> MSHPIQFVNANNSDKSHQLGGQYSIPQDLRENLQKEAARIGENEKDVLQEKMETRTVQNREDSYHKRRFDMKFEPDSDTQTVTSSENTQDAVVPRKRKSRWDVKGYEPPDESSTAVKENSDSALVNVEGIHDLMFFKPSDHKYFADVISKKPIDELNKDEKKERTLSMLLLKIKNGNTASRRTSMRILTDKAVTFGPEMIFNRLLPILLDRSLEDQERHLMIKTIDRVLYQLGDLTKPYVHKILVVAAPLLIDEDPMVRSTGQEIITNLSTVAGLKTILTVMRPDIENEDEYVRNVTSRAAAVVAKALGVNQLLPFINAACHSRKSWKARHTGIKIVQQIGILLGIGVLNHLTGLMSCIKDCLMDDHVPVRIVTAHTLSTLAENSYPYGIEVFNVVLEPLWKGIRSHRGKVLSSFLKAVGSMIPLMDPEYAGYYTTEAMRIIRREFDSPDDEMKKTILLVLQKCSAVESITPKFLREEIAPEFFQKFWVRRVALDRPLNKVVTYTTVTLAKKLGCSYTIDKLLTPLRDEAEPFRTMAVHAVTRTVNLLGTADLDERLETRLIDALLIAFQEQTNSDSIIFKGFGAVTVSLDIRMKPFLAPIVSTILNHLKHKTPLVRQHAADLCAILIPVIKNCHEFEMLNKLNIILYESLGEVYPEVLGSIINAMYCITSVMDLDKLQPPINQILPTLTPILRNKHRKVEVNTIKFVGLIGKLAPTYAPPKEWMRICFELLELLKSTNKEIRRSANATFGFIAEAIGPHDVLVALLNNLKVQERQLRVCTAVAIGIVAKVCGPYNVLPVIMNEYTTPETNVQNGVLKAMSFMFEYIGNMSKDYIYFITPLLEDALTDRDLVHRQTASNVITHLALNCSGTGHEDAFIHLMNLLIPNIFETSPHAIMRILEGLEALSQALGPGLFMNYIWAGLFHPAKNVRKAFWRVYNNMYVMYQDAMVPFYPVTPDNNEEYIEELDLVL;> MWGGGKMAVVSLSPHTAKMRKLFGQASTTMAYDGLKREAERRTRSDHNITMVAKDDELYLYHLTLKKQTNFVHSCIGHFVDLEAGSKREQSQLCVATETHLELYDTADGELKLIAKFQNLFATITSMKSLDLPHSGSRAKASNWPTFLALTSDSGNLSIVQIIMHAGALRLKTLVNQPLTRTTLRRVSPISYMEIDPNGRCIILSSVEQNKLCFLVDYAQKLRISSPLEIIRPHMVTLDMAVVDVNFNNPCFVTLEIDNAATQLSVHLIFYVLELGLNHIVKKADYLVNPSANFVLSLPDLSRYNITTSLSDNNYDADYDTLFNPFVVIGFENHILVKDMNGFFSLKVEIPKRSITNSRHKNVTIISGIVQKLKNDFFVLLQSNHGDLFKLTVSPDTNDRNRPLVQLSYFDTIQNSHQLHIFKNGYLFALSEMNNNFLFQFEKLGVEKNDFSNVLTSKDPNKSLVFEPSIKLQNLSILSQQLNLNPSIKSQIVSDSPLSIATKHFTNNKIITLTNAVNYSNLISTSLPPNATKLWLIPDPATTGDNNTLLFITFPKKTMILQIDNESMEELTPDEATRSAFKLSQDTTIHTCLMGSHSIIQVCTAELRHIVPTGKSRYSNKLTWVPPAGIRIVCATSSKTQLIISLSNYELVYFKIDVSSDSLIELTTHPELDTMPSKVAIVQDTQHADLLAIADNEGMIKIMSLKDQKEDFLTVISLQLVSEKISDMIMVRDSSIGQLNLHVGLENGVYMKFHIGDVDGSFTDIKRRFLGLKPVSLSYLREISVSLNNEEEEEEEEDDDDEKEEEEINSSGAKWMSCVVCHSSSTWVSYTWKNVWTIRQLKDQNMLSCSKFVNADVAINGVCSISSSGRLNIGRVSNFPTLDNWFHVHESSVNKQENGGGDESNEEEEDEMEEEMEMLQISTFRPRTILSFPNNPKSILFIDNHSGKKQCRISLQIDGECLKFGSSDHLYKILDDIDCVSAAIIDFTRQADHLIICAGDKRLLTYKILVNKDKLSFDIELLHQTEIISPIHAMLKFKNFLLTAMGSTIVLYGLGKKQLLRRSVTQTPVSITKIVSMHQWNYERLAVGDIHESVTLFIWDPAGNVFIPYVDDSVKRHVTVLKFLDEATVIGADRYGNAWTLRSPPECEKIMSNHDPSELSNGAIKYPLDVITLQQKLPNTYDCKFKFQLLNHFFVNDIITDFHILDSLSNSDRPGCIYMGLQGTVGCFIPLLSKGNVFMMGNIENIMAEADDTFYLDYESRKKNNNMRKEDDEEESGSVVLQGRHGIEDEIICEGSCSILGRDHQEYRSYYAPVRKVIDGDLCENFLRLSLNEQEFLAKNLKSVQVEDIIQTINEVRTNYM;> MARTKSRKRSGNNQNKNASVVNNKAEIAAMIDARRLEQKKKGGVTNSKGKTNKVVDAKLEKEFKDVLQRFQVQENDTPKEITKDEKNNHVVIVEKNPVMNRKHTAEDELEDTPSDGIEEHLSARKRRKTEKPSLSQLKSQVPYPQIIEWYDCDARYPGLLASIKCTKNVIPVPSHWQSKKEYLSGRSLLGKRPFELPDIIKKTNIEQMRSTLPQSGLDGQDEKSLKEASRARVQPKMGALDLDYKKLHDVFFKIGANWKPDHLLCFGDVYYENRNLFEETNWKRMVDHKRPGRISQELRAIMNLPEGQLPPWCMKMKDIGLPTGYPDLKIAGLNWDITNLKGDVYGKIIPNHHSRSKKQGRNYFGALISFETPEFENSKEDTQANAENGRQDDKIDDEVEHKLDHFQEDISEVTSAEEKLERNEEESEKQLYTVLK;> MNYSADSGNTVYVGNIDPRITKEQLYELFIQINPVLRIKYPKDKVLQAYQGYAFIEFYNQGDAQYAIKIMNNTVRLYDRLIKVRQVTNSTGTTNLPSNISKDMILPIAKLFIKNLADSIDSDQLVKIFNKFGKLIREPEIFYLSNGKLKCAYVYFEDFEKADLAIKSLNNQLVANNRITVDYAFKENGKGNAKYGDDVDRLLNKEALKHNMLK;> MSRHQFDLIMCLKQPGVQTGLLCEKCDGKCPICDSYVRPKRKVRVCENCSFGKQAKNCIICNLNVGVNDAFYCWECCRLGKDKDGCPRILNLGSNRLDRHFEKKKKV;> MNLLETRRSLLEEMEIIENAIAERIQRNPELYYHYIQESSKVFPDTKLPRSSLIAENKIYKFKKVKRKRKQIILQQHEINIFLRDYQEKQQTFNKINRPEETQEDDKDLPNFERKLQQLEKELKNEDENFELDINSKKDKYALFSSSSDPSRRTNILSDRARDLDLNEIFTRDEQYGEYMELEQFHSLWLNVIKRGDCSLLQFLDILELFLDDEKYLLTPPMDRKNDRYMAFLLKLSKYVETFFFKSYALLDAAAVENLIKSDFEHSYCRGSLRSEAKGIYCPFCSRWFKTSSVFESHLVGKIHKKNESKRRNFVYSEYKLHRYLKYLNDEFSRTRSFVERKLAFTANERMAEMDILTQKYEAPAYDSTEKEGAEQVDGEQRDGQLQEEHLSGKSFDMPLGPDGLPMPYWLYKLHGLDREYRCEICSNKVYNGRRTFERHFNEERHIYHLRCLGIEPSSVFKGITKIKEAQELWKNMQGQSQLTSIAAVPPKPNPSQLKVPTELELEEEDEEGNVMSKKVYDELKKQGLV;> MNYLEGVGSKKGGGGIASESQFNLQRRKEVESLLSKGENVPYTFQDEKDDQVRSNPYIYKNHSGKLVCKLCNTMHMSWSSVERHLGGKKHGLNVLRRGISIEKSSLGREGQTTHDFRQQQKXXXXXXXXXXXXXXXXIIEAKQSLKNNGTIPVCKIATVKNPKNGSVGLAIQVNYSSEVKENSVDSDDKAKVPPLIRIVSGLELSDTKQKGKKFLVIAYEPFENIAIELPPNEILFSENNDMDNNNDGVDELNKKCTFWDAISKLYYVQFFFKQAEQEQADV;> MEPEDTQLKEDIKTTVNYIKQHGVEFENKLLEDERFSFIKKDDPLHEYYTKLMNEPTDTVSGEDNDRKSEREIARPPDFLFSQYDTGISRRDMEVIKLTARYYAKDKSIVEQMISKDGEARLNFMNSSHPLHKTFTDFVAQYKRVYSFTGQEIKKSKRTILDNCFERTQYWEFEKDKDREHDKLVELCKIQFAAIPWDKFTQVAKFSIPEDTEIFEGSLDLEQMRLRRVQTGIKLFDSIKPTNEEEKIVSDQGKQKGGDSKGKKRKIRAVGETRLKKSKK;> MKFTPSIVIDAPQYYVDHFNGKYNVDKCVILRDLQLETDSESMPSSLKHLTKPTHILDLTNNDLIMIPDLSRRDDIHTLLLGRNNIVEVDGRLLPMNVQNLTLSNNSIRRFEDLQRLRRAPRTLKNLTLIGNQVCHLANYREHVLRLVPHLETLDFQNVTAEERKSAMSFPRQADGDTLGPVNTAIRDNGSRDKTMEIMNLVVSKMTVERRNELKKQLAEATSLEEIARLEKLLSGGV;> MVEPARKKQRIDRDTHHTVAEPVTEAKNTLYVSQLNEKINMQRLRVNLFLLFATFGEVLKVSMNFKKQRGQAFITMRTIDQASLAQISLNGERFFGKPLKVEFSKSETKTL;> MAEKQRQLKLQKIYKQKYIGLGDESTTREQWQRNVRNDTLNTLQGHSASLEYVSLSRGDLSIRDTRIHLLKSMSPGYKAYLREE;> METIDSKQNINRESLLEERRKKLAKWKQKKAQFDAQKEHQTSRNDIVTNSLEGKQTTEKFTERQERVKEELRKRKNEFRKSDEPVSVKPSKKKSKRSKVKKKISFDFSDDDDSEIGVSFRSKEHIQKAPEHDNEKDPLDEFMTSLKEEKMSNSKGMYDRGDILDVEDQLFELGGTDDEDVEDNTDNSNIAKIAKLKAKKRVKQIYYSPEELEPFQKNFYIESETVSSMSEMEVEELRLSLDNIKIKGTGCPKPVTKWSQLGLSTDTMVLITEKLHFGSLTPIQSQALPAIMSGRDVIGISKTGSGKTISYLLPLLRQVKAQRPLSKHETGPMGLILAPTRELALQIHEEVTKFTEADTSIRSVCCTGGSEMKKQITDLKRGTEIVVATPGRFIDILTLNDGKLLSTKRITFVVMDEADRLFDLGFEPQITQIMKTVRPDKQCVLFSATFPNKLRSFAVRVLHSPISITINSKGMVNENVKQKFRICHSEDEKFDNLVQLIHERSEFFDEVQSENDGQSSDVEEVDAKAIIFVSSQNICDFISKKLLNAGIVTCAIHAGKPYQERLMNLEKFKREKNSILLCTEVLSRGLNVPEVSLVIIYNAVKTFAQYVHTTGRTARGSRSGTAITLLLHDELSGAYILSKAMRDEEIKALDPLQAKELQEMSAKFESGMKKGKFRLSKGFGGKGLENIKSKREEAQNKDLELKKNDKRSDDLEKKISNPREGHDSVSESSALIPRLNYELFKESTDGSIIFYAKVYINDLPQIVRWEATKNTTLLFIKHETGCSITNKGKFYPEGKEPKNENDEPKLYLLIEGQDEKDIQLSIELLEQKVKEGVVKAASLSLKSTKY;> MSKIQVAHSSRLANLIDYKLRVLTQDGRVYIGQLMAFDKHMNLVLNECIEERVPKTQLDKLRPRKDSKDGTTLNIKVEKRVLGLTILRGEQILSTVVEDKPLLSKKERLVRDKKEKKQAQKQTKLRKEKEKKPGKIAKPNTANAKHTSSNSREIAQPSSSRYNGGNDNIGANRSRFNNEAPPQTRKFQPPPGFKRK;> MKLVNFLKKLRNEQVTIELKNGTTVWGTLQSVSPQMNAILTDVKLTLPQPRLNKLNSNGIAMASLYLTGGQQPTASDNIASLQYINIRGNTIRQIILPDSLNLDSLLVDQKQLNSLRRSGQIANDPSKKRRRDFGAPANKRPRRGL;> MSSQIIDRPKHELSRAELEELEEFEFKHGPMSLINDAMVTRTPVIISLRNNHKIIARVKAFDRHCNMVLENVKELWTEKKGKNVINRERFISKLFLRGDSVIVVLKTPVE;> MTMNGIPVKLLNEAQGHIVSLELTTGATYRGKLVESEDSMNVQLRDVIATEPQGAVTHMDQIFVRGSQIKFIVVPDLLKNAPLFKKNSSRPMPPIRGPKRR;> MSNKVKTKAMVPPINCIFNFLQQQTPVTIWLFEQIGIRIKGKIVGFDEFMNVVIDEAVEIPVNSADGKEDVEKGTPLGKILLKGDNITLITSA;> MSESSDISAMQPVNPKPFLKGLVNHRVGVKLKFNSTEYRGTLVSTDNYFNLQLNEAEEFVAGVSHGTLGEIFIRCNNVLYIRELPN;> MVSTPELKKYMDKKILLNINGSRKVAGILRGYDIFLNVVLDDAMEINGEDPANNHQLGLQTVIRGNSIISLEALDAI

Here, by deleting the branch-site adenosine (BS-A) or mutating the branch-site sequence of an actin pre-mRNA, we stall the assembly of spliceosomes in extracts from the yeast Saccharomyces cerevisiae directly before the A complex is formed. We then determine the three-dimensional structure of this newly identified assembly intermediate by cryo-electron microscopy. Our structure indicates that the U2–BS helix has formed in this pre-A complex, but is not yet clamped by the HEAT domain of the Hsh155 protein (Hsh155HEAT), which exhibits an open conformation. Thus, Prp5 proofreads the branch site indirectly, hindering spliceosome assembly if branch-site mutations prevent the remodelling of Hsh155HEAT.

Further classification and multibody refinement improved the resolution of the stable U1 snRNP region and adjacent U2 5′ region to 4.1 Å and 8.3 Å, respectively. Stem–loop (SL) IIa of U2 snRNA is bound by Hsh155, Cus1 and Prp9 in the ΔBS-A complex, in a similar manner to that seen in the human 17S U2 snRNP and subsequently formed spliceosomal complexes. An extended helical density element is located directly upstream of SLIIa. This element is longer than the U2 branchpoint-interacting stem-loop (BSL), which is found in the isolated U2 snRNP and sequesters U2 nucleotides that base pair with the branch site. A modelled, extended U2–BS helix—lacking a bulged BS-A and comprising 13 base pairs—fits well into this density element, indicating that an extended U2–BS helix has formed. In the ΔBS-A complex, the U2–BS helix is located further away from the carboxy (C)-terminal HEAT repeats of Hsh155HEAT compared with its position in the A to Bact complexes, and it is not sequestered by Hsh155HEAT. We find here that, in the yeast pre-A complex, Cus2 (human TAT–SF1) has dissociated and the Prp5RecA domains are located between the U2 3′-region and the U2–BS helix. Compared with their position in 17S U2 snRNP, the Prp5RecA domains in the pre-A complex are located further away from Hsh155HEAT, with RecA1 fitting well into the niche formed by the amino (N)-terminal region of Prp9 (Prp9NTR), with which it interacts, and the U2–BS helix. Moreover, Prp5RecA1 now contacts the U2 snRNA strand that connects SLIIa and the U2–BS helix.>GSHMGQDIQLIPP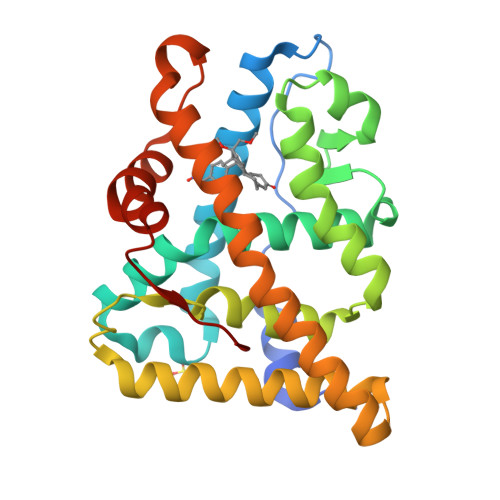LINLLMSIEPDVIYAGHDNTKPDTSSSLLTSLNQLGERQLLSVVKWSKSLPGFRNLHIDDQITLIQYSWMSLMVFGLGWRSYKHVSGQMLYFAPDLILNEQRMKESSFYSLCLTMWQIPQEFVKLQVSQEEFLCMKVLLLLNTIPLEGLRSQTQFEEMRSSYIRELIKAIGLRQKGVVSSSQRFYQLTKLLDNLHDLVKQLHLYCLNTFIQSRALSVEFPEMMSEVIAAQLPKILAGMVKPLLFHKK[2x]>[6x]MDKDCEMKRTTLDSPLGKLELSGCEQGLHEIKLLGKGTSAADAVEVPAPAAVLGGPEPLMQATAWLNAYFHQPEAIEEFPVPALHHPVFQQESFTRQVLWKLLKVVKFGEVISYQQLAALAGNPAATAAVKTALSGNPVPILIPCHRVVSSSGAVGGYEGGLAVKEWLLAHEGHRLGKPGLGPAGYPYDVPDYAYPYDVPDYAYPYDVPDYAGSSGLEVLFQGPTVEKEAPDAHFTVDKQNISLWPREPPPKSGPSLVPGKTPTVRAALICLTLVLVASVLLQAVLYPRFMGTISDVKTNVQLLKGRVDNISTLDSEIKKNSDGMEAAGVQIQMVNESLGYVRSQFLKLKTSVEKANAQIQILTRSWEEVSTLNAQIPELKSDLEKASALNTKIRALQGSLENMSKLLKRQNDILQVVSQGWKY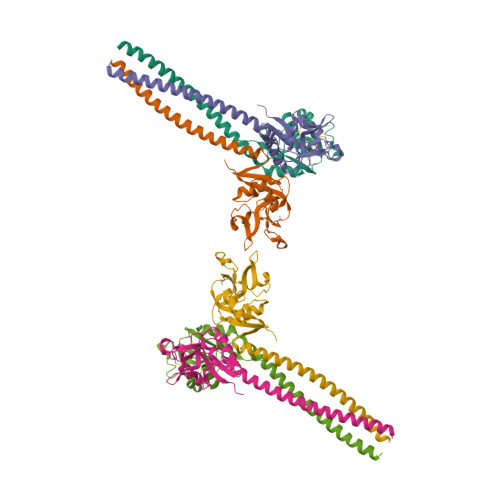FKGNFYYFSLIPKTWYSAEQFCVSRNSHLTSVTSESEQEFLYKTAGGLIYWIGLTKAGMEGDWSWVDDTPFNKVQSARFWIPGEPNNAGNNEHCGNIKAPSLQAWNDAPCDKTFLFICKRPYVPSEP>MFNMNVDESASGALGSSAIPVHPTPASVRLFEILQGKYAYVQGQTIYANLRNPGVFSRQVFTHLFKRAISHCTYDDVLHDWNKFEACIQKRWPSDDSCASRFRESTFESWSTTMKLTVRDLLTTNIYRVLHSRSVLSYERYVDWICATGMVPAVKKPITQELHSKIKSLRDRCVCRELGHERTIRSIGTELYEATKEIIESLNSTFIPQFTEVTIEYLPRSDEYVAYYCGRRIRLHVLFPPAIFAGTVTFDSPVQRLYQNIFMCYRTLEHAKICQLLNTAPLKAIVGHGGRDMYKDILAHLEQNSQRKDPKKELLNLLVKLSENKTISGVTDVVEEFITDASNNLVDRNRLFGQPGETAAQGLKKKVSNTVVKCLTDQINEQFDQINGLEKERELYLKKIRSMESQLQASLGPGGNNPAASAPAAVAAEAASVDILTGSTASAIEKLFNSPSASLGARVSGHNESILNSFVSQYIPPSREMTKDLTELWESELFNTFKLTPVVDNQGQRLYVRYSSDTISILLGPFTYLVAELSPVELVTDVYATLGIVEIIDELYRSSRLAIYIEDLGRKYCPASATGGDHGIRQAPSARG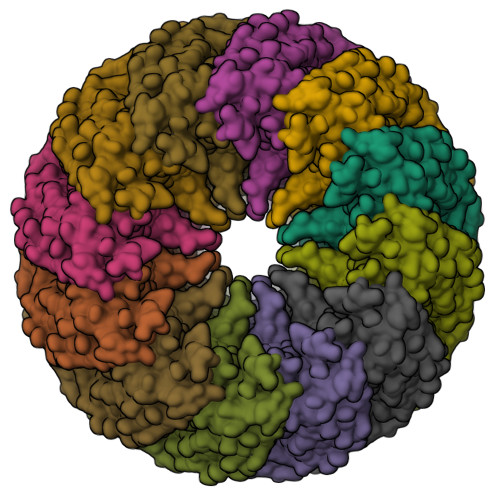DTEPDHAKSKPARDPPPGAGS[12x]> QNQIVSGAAWTDTAGNTIQAHGAGILQVGSTFYWFGEDKSHNSALFKAVSCYTSSD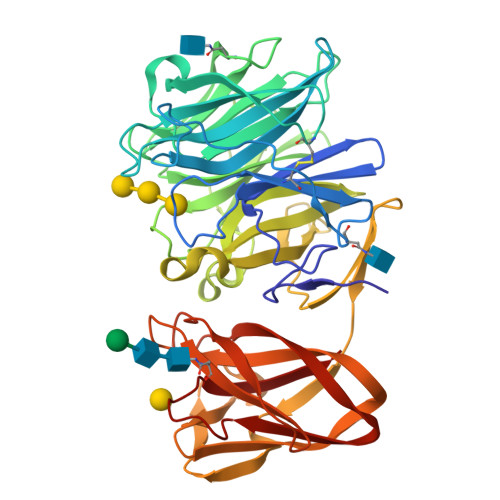LVNWSRQNDALSPIAGTMISTSNVVERPKVIFNQKNSEYVMWFHSDSSNYGAAMVGVATAKTPCGPYTYKGSFKPLGADSRDESIFQDDDSAQTAYLLYASDNNQNFKISRLDANYYNVTAQVSVMNGATLQAPGIVKHNGEYFLIASHTSGWAPNPNKWFSASSLAGPWSAQQDIAPSATRTWYSQNAFDLPLGSNAIYMGDRWRPSLLGSSRYIWYPLDFSSGAPQIVHADVWSVNVQAGTYSVASGTSYEAENGQRGGSSTILSGSGFSGGKAVGYLGHGGTVTINNVQSNGGSHWVALYFANGDSTYRNVTVSVNGGPSVLVDQPDSGGGNVVISVPVKLNLNSGENSITFGSGQSNYAADLDKIIVY>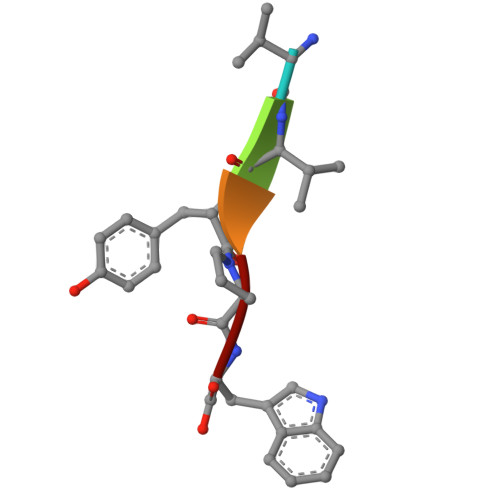 VVYPW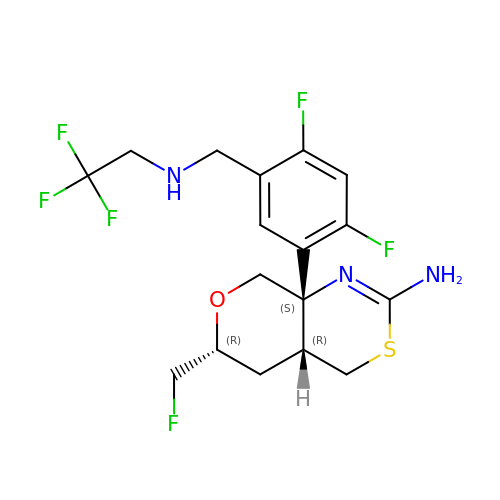(4aR,6R,8aS)-8a-(2,4-difluoro-5-{[(2,2,2-trifluoroethyl)amino]methyl}phenyl)-6-(fluoromethyl)-4,4a,5,6,8,8a-hexahydropyrano[3,4-d][1,3]thiazin-2-amine | C17 H19 F6 N3 O S | KXRWMDHPUURSND-USBNGQNGSA-N>[2x]MGSDKIHHHHHHMKRILVSLYEKEKYLDILRELHEKGWEIWASSGTAKFLKSNGIEANDVSTITGFENLLGGLVKTLHPEIFAGILGPEPRWDVVFVDLYPPPDIDIGGVALLRAAAKNWKKVKPAFDMETLKLAIEIDDEETRKYLAGMTFAFTSVYDSIRANQFVEGISLAFKREDLQLRYGENPH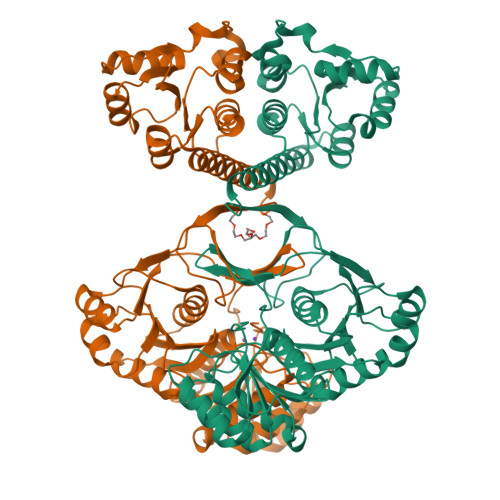EKAFVYGKPAFEILHEGKTISFNNILDAENAWFMAKNLPRMGAVVVKHQSPCGAAIGEDKVEIVKKAIEADDESSFGGILAVNFEMDEEVAKSLKKYLEVIVAPSFTQEAIEVLSKKKVRLLKPGDYASWAGKMAFGSLVLSERKYPEGNFELVVGEPLSEKELEDLEFAYRVVEGAKSNAVLIAKDGVTVGIGSGQPSRKRAAWIATVMAGEKAKGAVAASDAFFPFPDSLEILAQAGVKAVVAPLGSIRDEEVIEKARELGITFYKAPSRVFRH> 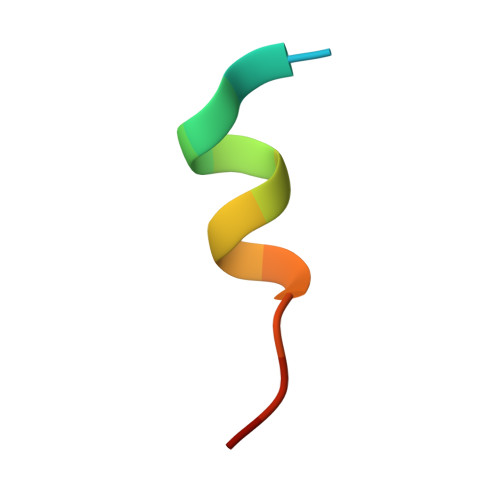SQETFSDLWKLLPEN> MENTENSVDSKSIKNLEPKIIHGSESMDSGISLDNSYKMDYPEMGLCIIINNKNWHKSTGMTSRSGTDVDAANLRETFRNLKYEVRNKNDLTREEIVELMRDVSKEDHSKRSSFVCVLLSHGEEGIIFGTNGPVDLKKITNFFRGDRCRSLTGKPKLFIIQACRGTELDCGIETDSGVDD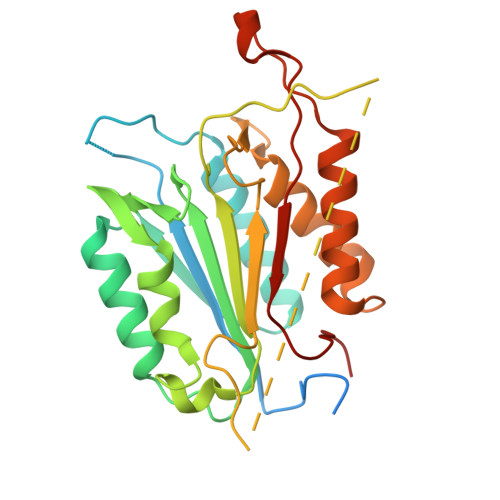DMACHKIPVEADFLYAYSTAPGYYSWRNSKDGSWFIQSLCAMLKQYADKLEFMHILTRVNRKVATEFESFSFDATFHAKKQIPCIVSMLTKELYFYHL>[3x]GPMGFVPETEDMLPRLAPRPSAAVPMGHTNEIIGPTVPEVSILFGQPPQDKAATPPPAANSSSDFKREITNADGSKDIWYPNGNLKKISADGMNLRMLYFNKDIKETNIREGTVKYYYAETNTWHTSYLDGLEILEFPNGQTEHRRKDGTVEIHFPNNSIKIVDPSDTEKLEEWRYADGTHLVQLRNGDKILNLPNGQKEIHTKLNKRRE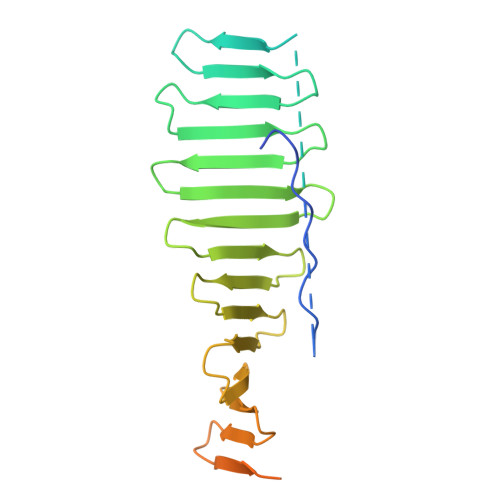YPDGTVKLVYPDGSQETRYSNGRVRLKDKDGKLIMDTDYAKY> MEPPTVALTVPAAALLPDGALGESIVRGRRYLSDTPAQLPDFVGNGLACRHCHPGRDGEVGTEANAAPFVGVVGRFPQYSARHGRLITLEQRIGDCFERSLNGRALALDHPA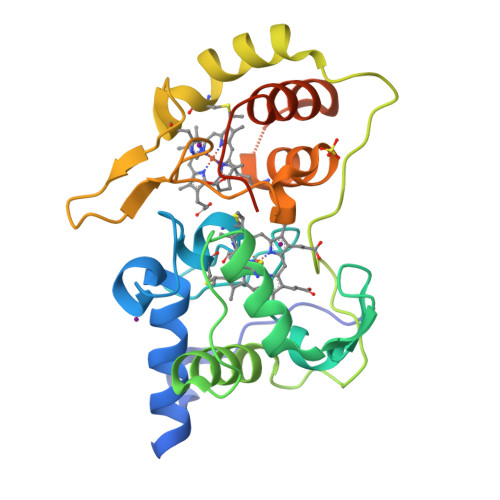LIDMLAYMSWLSQGVPVGAVVAGHGIPTLTLEREPDGVHGEALYQARCLACHGADGSGTLDADGRYLFPPLWGPRSFNTGAGMNRQATAAGFIKHKMPLGADDSLSDEEAWDVAGFVLTHPRPLFQEPTGDAWSHPQFEK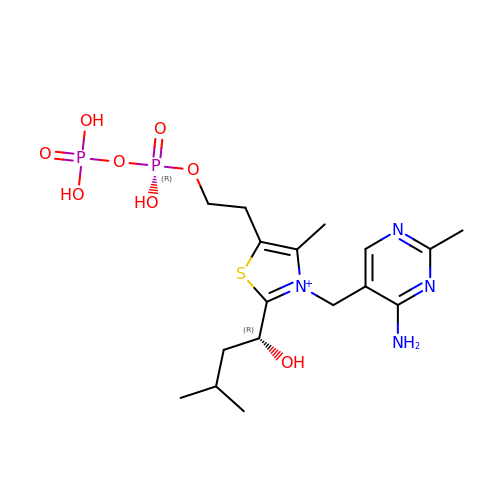C2-1-HYDROXY-3-METHYL-BUTYL-THIAMIN | C17 H29 N4 O8 P2 S | OZAWOYZVNPQFFO-CQSZACIVSA-O> DPISNAIENAVSTLADTTISRVTAANTAASSHSLGTGRVPALQAAETGASSNASDENLIETRCVMNRNGVNEASVEHFYSRAGLVGVVEVKDSGTSQDGYTVWPIDVMGFVQQRRKLELSTYMRFDAEFTFVSNLNDSTTPGMLLQYMYVPPGAPKPDGRKSYQWQTATNPSIFAKLSDPPPQVSVPFMSPASAYQWFYDGYPTFGEHKQATNLQYGQCPNNMMGHFAIRTVSESTTGKNVHVRVYMRIKHVRAWVPRPFRSQAYMVKNYPTYSQTISNTAADRASITTTDYEGGVPANPQRTF;> SPSVEACGYSDRVAQLTVGNSTITTQEAANIVLSYGEWPGYCPSTDATAVDKPTRPDVSVNRFYTLSTKSWKTESTGWYWKFPDVLNDTGVFGQNAQFHYLYRSGFCMHVQCNASKFHQGALLVVVIPEFVVAASSPATKPNGQGLYPDFAHTNPGKEGQVFRDPYVLDAGIPLSQALVFPHQWINLRTNNCATIIMPYVNALPFDSALNHSNFGLAVIPISPLKYCNGATTEVPITLTIAPLNSEFSGLRQAIKQ;> GLPTELKPGTNQFLTTDDGTSPPILPGFEPTPLIHIPGEFTSLLDLCRIETILEVNNTTGTTGVNRLLIPVRAQNNVDQLCASFQVDPGRNGPWQSTMVGQICRYYTQWSGSLKVTFMFTGSFMATGKMLIAYTPPGSAQPTTREAAMLGTHIVWDFGLQSSVTLVIPWISNTHFRAVKTGGVYDYYATG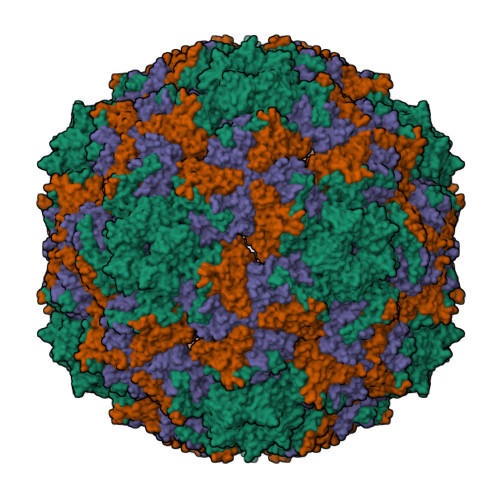IVTIWYQTNFVVPPDTPSEANIIALGAAQENFTLKLCKDTDEIRQTAEYQN>MAKKTSSKGKLPPGPTPLPFIGNYLQLNTEQMYNSLMKISERYGPVFTIHLGPRRVVVLCGHDAVREALVDQAEEFSGRGEQATFDWVFKGYGVVFSNGERAKQLRRFSIATLRDFGVGKRGIEERIQEEAGFLIDALRGTGGANIDPTFFLSRTVSNVISSIVFGDRFDYKDKEFLSLLRMMLGIFQFTSTSTGQLYEMFSSVMKHLPGPQQQAFQLLQGLEDFIAKKVEHNQRTLDPNSPRDFIDSFL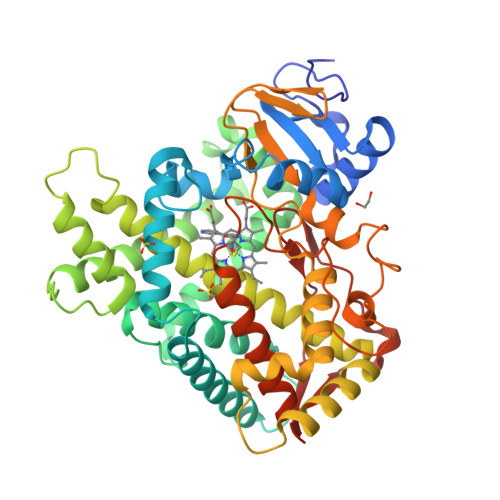IRMQEEEKNPNTEFYLKNLVMTTLNLFIGGTETVSTTLRYGFLLLMKHPEVEAKVHEEIDRVIGKNRQPKFEDRAKMPYMEAVIHEIQRFGDVIPMSLARRVKKDTKFRDFFLPKGTEVYPMLGSVLRDPSFFSNPQDFNPQHFLNEKGQFKKSDAFVPFSIGKRNCFGEGLARMELFLFFTTVMQNFRLKSSQSPKDIDVSPKHVGFATIPRNYTMSFLPRHHHH[4x]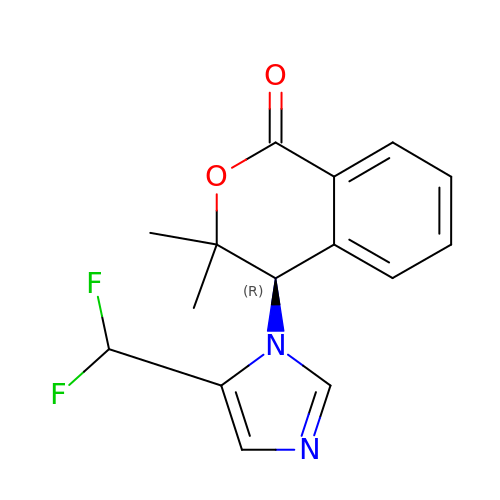(4R)-4-[5-(difluoromethyl)-1H-imidazol-1-yl]-3,3-dimethyl-3,4-dihydro-1H-2-benzopyran-1-one | C15 H14 F2 N2 O2 | LAMQMSRGFJHTEW-GFCCVEGCSA-N>EDVEIKPRGYQLRLVDHLTKSNGIVYLPTGSGKTFVAILVLKRFSQDFDKPIESGGKRALFMCNTVELARQQAMAVRRCTNFKVGFYVGEQGVDDWTRGMWSDEIKKNQVLVGTAQVFLDMVTQTYVALSSLSVVIIDECHHGTGHHPFREFMRLFTIANQTKLPRVVGLTGVLIKGNEITNVATKLKELEITYRGNIITVSDTKEMENVMLYATKPTEVMVSFPHQEQVLTVTRLISAEIEKFYVSLDLMNIGVQPIRRSKSLQCLRDPSKKSFVKQLFNDFLYQMKEYGIYAASIAIISLIVEFDIKRRQAETLSVKLMHRTALTLCEKIRHLLVQKLQDMTYDDDDDNVNTEEVIMNFSTPKVQRFLMSLKVSFADKDPKDICCLVFVERRYTCKCIYGLLLNYIQSTPELRNVLTPQFMVGRNNISPDFESVLERKWQKSAIQQFRDGNANLMICSSVLEEGIDVQACNHVFILDPVKTFNMYVQSKGRARTTEAKFVLFTADKEREKTIQQIYQYRKAHNDIAEYLKDRVLEKTEPELYEIKGHFQDDIDPFTNENGAVLLPNNALAILHRYCQTIPTDAFGFVIPWFHVLQEDERDRIFGVSAKGKHVISINMPVNCMLRDTIYSDPMDNVKTAKISAAFKACKVLYSLGELNERFVPKTLKERVASIADVHFEHWNKYGDSVTATVNKADKSKDRTYKTECPLEFYDALPRVGEICYAYEIFLEPQFESCEYTEHMYLNLQTPRNYAILLRNKLPRLAEMPLFSNQGKLHVRVANAPLEVIIQNSEQLELLHQFHGMVFRDILKIWHPFFVLDRRSKENSYLVVPLILGAGEQKCFDWELMTNFRRLPQSHGSNVQQREQQPAPRPEDFEGKIVTQWYANYDKPMLVTKVHRELTPLSYMEKNQQDKTYYEFTMSKYGNRIGDVVHKDKFMIEVRDLTEQLTFYVHNRGKFNAKSKAKMKVILIPELCFNFNFPGDLWLKLIFLPSILNRMYFLLHAEALRKRFNTYLNLHLLPFNGTDYMPRPLEIDYSLKRNVDPLGNVIPTEDIEEPKSLLEPMPTKSIEASVANLEITEFENPWQKYMEPVDLSRNLLSTYPVELDYYYHFSVGNVCEMNEMDFEDKEYWAKNQFHMPTGNIYGNRTPAKTNANVPALMPSKPTVRGKVKPLLILQKTVSKEHITPAEQGEFLAAITASSAADVFDMERLEILGNSFLKLSATLYLASKYSDWNEGTLTEVKSKLVSNRNLLFCLIDADIPKTLNTIQFTPRYTWLPPGISLPHNVLALWRENPEFAKIIGPHNLRDLALGDEESLVKGNCSDINYNRFVEGCRANGQSFYAGADFSSEVNFCVGLVTIPNKVIADTLEALLGVIVKNYGLQHAFKMLEYFKICRADIDKPLTQLLNLELGGKKMRANVNTTEIDGFLINHYYLEKNLGYTFKDRRYLLQALTHPSYPTNRITGSYQELEFIGNAILDFLISAYIFENNTKMNPGALTDLRSALVNNTTLACICVRHRLHFFILAENAKLSEIISKFVNFQESQGHRVTNYVRILLEEADVQPTPLDLDDELDMTELPHANKCISQEAEKGVPPKGEFNMSTNVDVPKALGDVLEALIAAVYLDCRDLQRTWEVIFNLFEPELQEFTRKVPINHIRQLVEHKHAKPVFSSPIVEGETVMVSCQFTCMEKTIKVYGFGSNKDQAKLSAAKHALQQLSKCDA[3x];> IDRYEQVSKDFEFIKI;>MEESMEELEALRRKKFTTYWELKEAGSVDHTGMRLCDRHNYF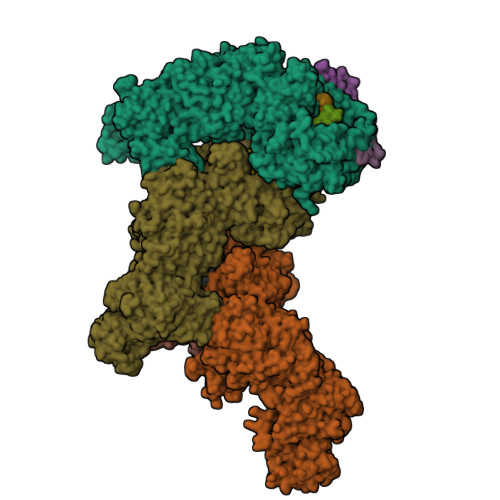KNFYPTLKKEAIEAINSDEYESSKDKAMDVMSSLKITPKISEVESSSLVPLLSVELNCAFDVVLMAKETDIYDHIIDYFRTMLI[3x]> K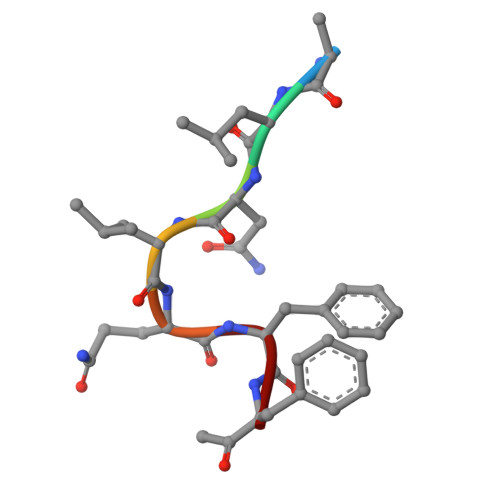LNLQFF>MKSVLILAGLVAVALSSAVPKPSTIKTKNVDAVFVEKQKKILSFFQDVSQLNTDDEYYKIGKDYDIEMNMDNYTNKKAVEEFLKMYRTGFMPKNLEFSVFYDKMRDEAIALFHLFYYAKDFETFYKTACFARVHLNQGQFLYAFYIAVIQRSDCHGFVVPAPYEVYPKMFMNMEVLQKIYVTKMQDGLINPEAAAKYGIHKENDY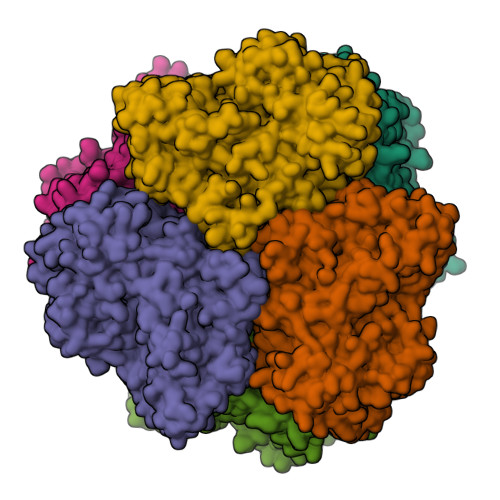FVYKANYSNAVLYNNEEQRLTYFTEDIGMNAYYYYFHSHLPFWWTSEKYGALKERRGEVYFYFYQQLLARYYFERLTNGLGKIPEFSWYSPIKTGYYPLMLTKFTPFAQRPDYYNLHTEENYERVRFLDTYEKTFVQFLQKDHFEAFGQKIDFHDPKAINFVGNYWQDNADLYGEEVTKDYQRSYEVFARRVLGAAPMPFDKYTFMPSAMDFYQTSLRDPAFYQLYNRIVEYIVEFKQYLKPYTQDKLYFDGVKITDVKVDKLTTFFENFEFDASNSVYFSKEEIKNNHVHDVKVRQPRLNHSPFNVNIEVDSNVASDAVVKIFLAPKYDDNGIPLTLEDNWMKFFELDWFTTKLTAGQNKIIRNSNEFVIFKEDSVPMTEIMKMLDEGKVPFDMSEEFCYMPKRLMLPRGTEGGFPFQLFVFVYPFDNKGKDLAPFESFVLDNKPLGFPLDRPVVDALFKVPNMYFKDIFIYHEGERFPYKFNIPSYDTQSNVVPKN[3x];>[3x]MKTVLILAGLIALALSSTVPEFKTTPVDAAFVEKQKKILSLFYNVNEISYEAEYYKVAQDFNIEASKDCYTNMKAYENFMMMYKVGFLPKNLEFSIFYEKMREEAIALFKLFYYAKDFECFYKTACYARVYMNQGMFLYAYYIAIIQRSDTASFVLPAPYEAYPQYFVNMEVKNKMDYVKMMDGCLDEKICYNYGIIKENEQFVMYANYSNSLTYPNNEDRIAYLTEDVGLNAYYYYFHSHLPFWWNSGKYGAFKERRGEIYFFFYQQLLARYYMERLTNGLGKIPEFSWYSPLRTGYLPPFNSFYYPFAQRSNDYELHTEKNYEEIRFLDIYEKTFFQYLQQGHFKAFDKKIDLHSSKAVNFVGNYWQTNADLFEEDFLQFYQRSYEVNARRVLGAAPKPFNQYTFIPSALDFYQTSARDPAFYQLYKRIVQYIIEFKQYQVPYTQEALHFVGLKISDVKVDKMVTFFDHFDFDAFNTVYFSKEELKSSPHGYKVRQPRLNHKPFTVTIDIKSDVATNAVVKMFLGPKYDENGFPFSLEDNWMNFYELDWFVQKVNPGQSQITRSSTDFAFFKEDSLPMAEIYKLLDQGKIPTDMFNSSDTMPSRLMLPKGTYDGFPFQLFVFVYPYEPTPKESEPFKAVVPDNKPFGYPFDRPVLPQYFKQPNMFFKKVLVYHEGELFPYLFNIPHYTPDKAQL N-[(benzyloxy)carbonyl]-D-tyrosyl-L-phenylalanyl-L-tyrosine | C35 H35 N3 O8 | 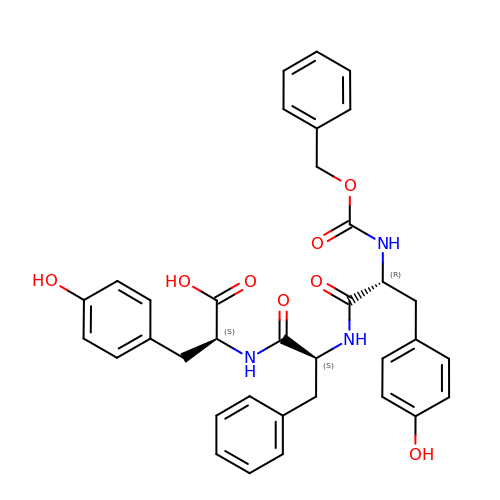NYJFXELTSYMIOY-YPKYBTACSA-N>MASRGVNKVILVGNLGQDPEVRYMPSGGAVANFTLATSESWRDKQTGEMKEQTEWHRVVLFGKLAEVAGEYLRKGSQVYIEGQLRTRKWTDQSGQDKYTTEVVVNVGGTMQMLGGRQGGGAPAGGGQQQGGWGQPQQPQGGNQFSGGAQSRPQQQAPAAPSNEPPMDFDDDIPFHHHHHH[4x]

Single-stranded DNA (ssDNA)-binding proteins (SSBs) play crucial roles in DNA replication, repair, recombination, and replication fork restart in both prokaryotes and eukaryotes. SSB binds to ssDNA with high affinity, regardless of sequence, and prevents premature annealing, chemical attacks, and unwanted nuclease digestion. SSBs typically recognize ssDNA via a highly conserved oligonucleotide/oligosaccharide-binding (OB) fold formed from a five-stranded β-barrel capped by an α-helix. SSB consists of an N-terminal ssDNA-binding/oligomerization domain (SSBn) and a flexible C-terminal protein–protein interaction domain (SSBc).

We crystallized KpSSB through hanging drop vapor diffusion and determined its structure at a resolution of 2.35 Å. Four monomers of KpSSB per asymmetric unit were present. The KpSSB monomer has an OB-fold domain similar to EcSSB, and the core of the OB-fold domain possesses a β-barrel capped with an α-helix. Unlike Streptomyces coelicolor SsbB, Staphylococcus aureus SsbA (SaSsbA) and SaSsbB, KpSSB contained additional β6 strand. β6 strands function by clamping two neighboring subunits together in a tetrameric SSB. The amino acids 120–174 in the structure of KpSSB were not observed, suggesting that the C-terminal region in KpSSB was dynamic, similar to that in EcSSB. Many hydrogen bonds and salt bridges were formed at the dimer–dimer interface of KpSSB. As compared with the crystal structures of the EcSSB- and Pseudomonas aeruginosa SSB (PaSSB)–ssDNA complex, we found that a GGRQ motif occurs at residues 114, which might be a regulatory switch for SSBn or ssDNA binding. In the structure of KpSSB, the GGRQ motif interacted with Asn14, Lys74, and Gln77 via several hydrogen bonds. These GGRQ motif-interacting residues (Asn14, Lys74, and Gln77) in KpSSB, perfectly conserved in EcSSB and PaSSB, are ssDNA-binding residues in EcSSB- and PaSSB–ssDNA complexes. Superimposing analysis indicated that if binding of the EcSSB–ssDNA complex occurs, the GGRQ peptide in KpSSB will break free from several hydrogen bonds and shift away by a distance of 12.2 Å and angles of 130˚ to form a complex with ssDNA.> MAEEGSSTKDSESFSVLNWDQVSRLHEVLTEVVPIHGRGNFPTLEITLKDIVQTVRGRLEEAGINVQDVRLNGSAAGHVLVKDNGLGCKDLDLIFHVALPTEAEFQLVRDVVLCSLLNFLPEGVNKLKISPVTLKEAYVQKLVKVCTDTDRWSLISLSNKNGRNVELKFVDSIRRQFEFSVDSFQIILDSLLFFYDCSGNPISEHFHPTVIGESMYGDFEEAFDHLQNRLIATKNPEEIRGGGLLKYSNLLVRDFRPADQEEIKTLER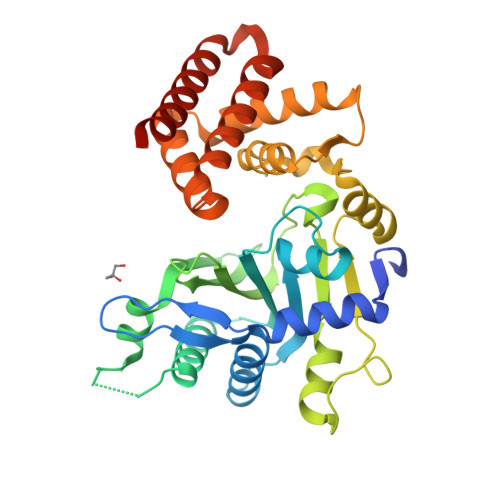YMCSRFFIDFPDILEQQRKLETYLQNHFSDEERSKYDYLMILRRVVNESTVCLMGHERRQTLNLISLLALRVLAEQNIIPS>[4x]GAMAPTPTDKHGGSDTRCPLMVKILD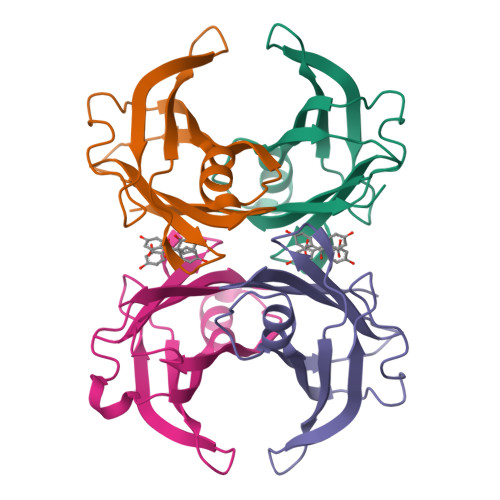AVKGTPAGSVALKVSQKTADGGWTQIATGVTDATGEIHNLITEQQFPAGVYRVEFDTKAYWTNQGSTPFHEVAEVVFDAHPEGHRHYTLALLLSPFSYTTTAVVSSVHE> RV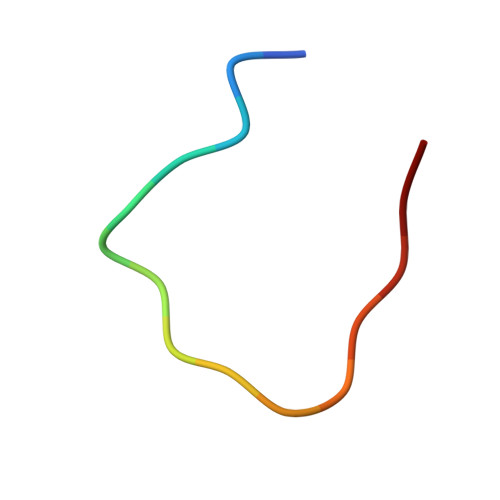WYPYGSYLTASGS> KGGAK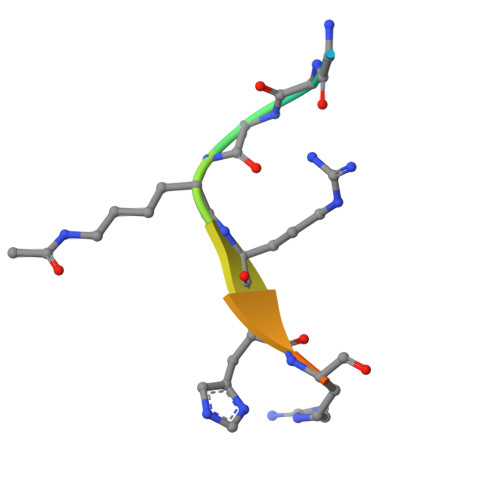RHRKIL> MDYKDDDDKHHHHHHTENLYFQGMATVEPETTPTPNPPTTEEEKTESNQEVANPEHYIKHPLQNRWALWFFKNDKSKTWQANLRLISKFDTVEDFWALYNHIQLSSNLMPGCDYSLFKDGIEPMWEDEKNKRGGRWLITLNKQQRRSDLDRFWLETLLCLIGESFDDYSDDVCGAVVNVRAK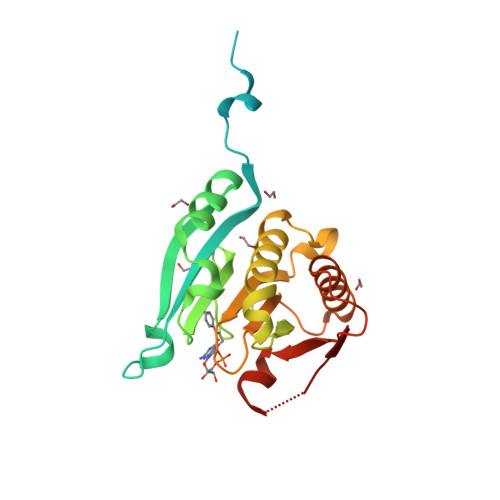GDKIAIWTTECENREAVTHIGRVYKERLGLPPKIVIGYQSHADTATKSGSTTKNRFVV5-BROMONICOTINAMIDE | C6 H5 Br 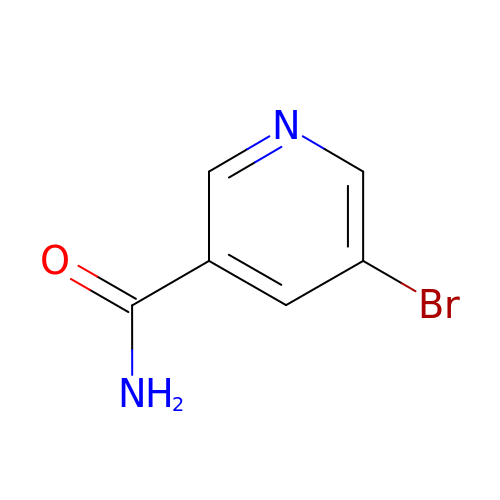N2 O | YOQRXZIMSKLRCY-UHFFFAOYSA-N>AECSVDIQGNDQMQFNTNAITVDKSCKQFTV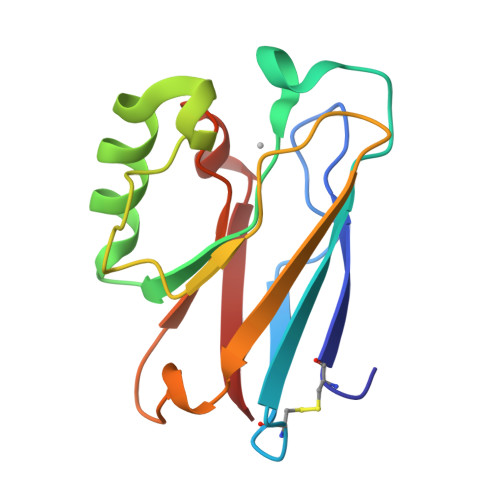NLSHPGNLPKNVMGHNWVLSTAADMQGVVTDGMASGLDKDYLKPDDSRVIAHTKLIGSGEKDSVTFDVSKLKEGEQYMFFCTFPGHSALMKGTLTLK[4x]> MTKLLDGKVAFITGSASGIGLEIAKKFAQEGAKVVISDMNAEKCQETANSLKEQGFDALSAPCDVTDEDAYKQAIELTQKTFGTVDILINNAGFQHVAPIEEFPTAVFQKLVQVMLTGAFIGIKHVLPIMKAQKYGRIINMASINGLIGFA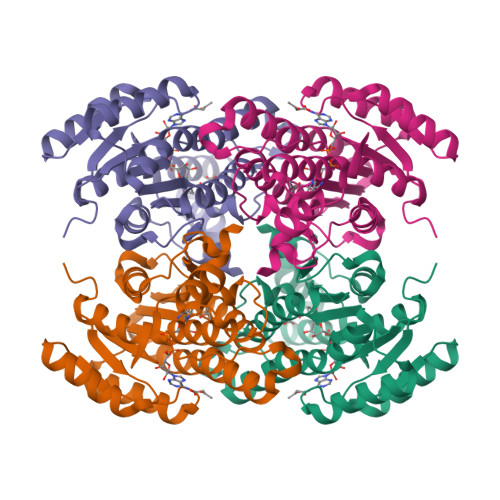GKAGYNSAKHGVIGLTKVAALECARDGITVNALCPGYVDTPLVRGQIADLAKTRNVSLDSALEDVILAMVPQKRLLSVEEIADYAIFLASSKAGGVTGQAVVMDGGYTAQ>SHMGQGGSNPKFENIAEGLRALLARSHVERTTDEGTWVAGVFVY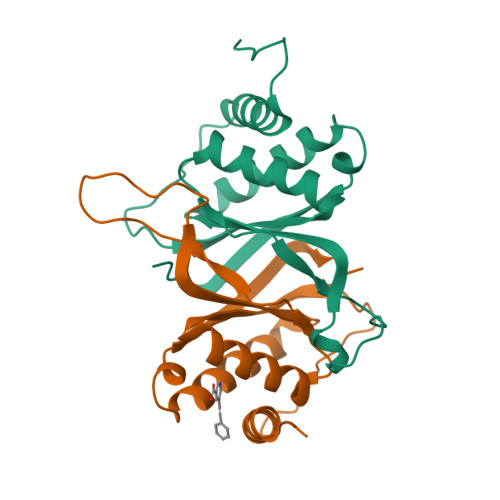GGSKTSLYNLRRGTALAIPQCRLTPLSRLPFGMAPGPGPQPGPLRESIVCYFMVFLQTHIFAEVLKDAIKDLVMTKPAPTCNIRVTVCSFDDGVDLP[2x]> KETKNVPFKLKNAAPVIFSHDIHLKKYNNNCRICHIALFDLRKPKRYTMLDMEKGKSCGACHTGMKAFSVADDSQCVRCHSGSARPVAYRMKG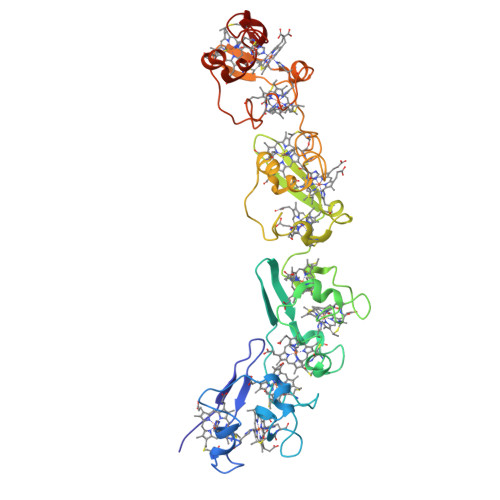AGEAVFSHEVHVPMLEGKCRTCHSNREITGGRNVTMAQMEKGKSCGACHNDKMAFTVAGNCGKCHKGMTPPKTVNFKMKGVADAAFSHEFHLGMYKCNECHTKLFAYKAGAKRFTMADMDKGKSCGACHNGKDAFSSASDCGKCHPGLKPAKLTYKTSVGEAYFDHDIHLSMFKCADCHTKVFKYRKGSAPATMADMEKGKSCGVCHNGKDAFSVADDCVKCHNM> MFLTAEDCFELGKVAYTEADYYHTELWMEQALRQLDEGE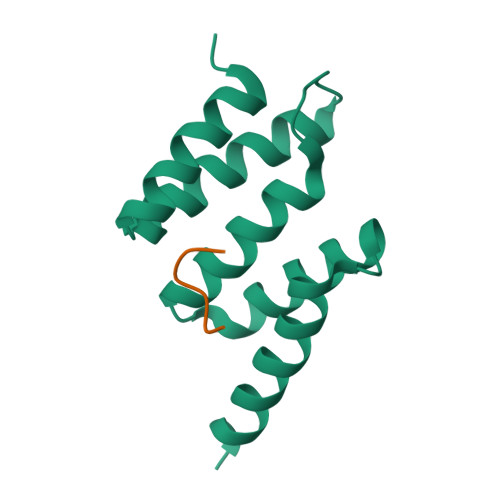ISTIDKVSVLDYLSYAVYQQGDLDKALLLTKKLLELDPEHQRANGNLKYFEYIMAKEKDVNKSAS;> HHHHHH> SRVLLALHDRAPQLKISDDRLTVVGEKGYSMVRASHGVRKGAWYFEITVDEMPPDTA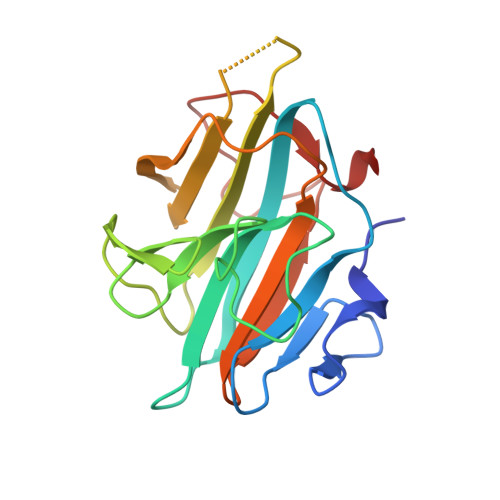ARLGWSQPLGNLQAPLGYDKFSYSWRSKKGTKFHQSIGKHYSSGYGQGDVLGFYINLPEDTISGRGSSEIIFYKNGVNQGVAYKDIFEGVYFPAISLYKSCTVSINFGPCFKYPPKDLTYRPMSDMG>MPGRRKACFVTALTSRTELDIDPDKLRESVVELLERHPLVFEGTRQLALQHRPEATDPWYEGCQRQSLISSDSDFTEVHGELRDTYLGEVFDRLPFKPIRTRIMALDPKYCYSVHRDLTPRYHLAVTTSEHARFVFIEHDKVLHIPADGDLYYVDTRQLH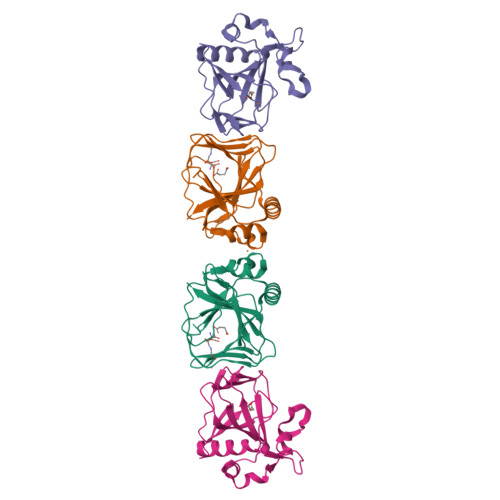SAFNGGDDMRIHIVFGTDGESK[2x]Recently, the novel multifunctional S-adenosyl-1-methionine (SAM)-dependent enzyme LepI, located in the PKS-NRPS gene cluster for leporin biosynthesis, was characterized in Aspergillus flavus. LepI is considered as a SAM-dependent methyltransferase that can catalyze stereoselective dehydration via three pericyclic transformational processes: intramolecular Diels-Alder and hetero-Diels-Alder reactions and a retro-Claisen rearrangement. The overall structure was found to be largely similar to that of SAM-dependent enzymes,28–31 exhibiting a core α/β fold of alternating β strands (β1–β7) and α helices (α1–α19). This structure exhibiting α helices and β sheets comprises an all-helix amino-terminal domain (NTD), a carboxy-terminal domain including a substrate-binding site, and a SAM-binding site, which is formed by a seven-stranded β sheet rounded with five helices.

To better understand the mechanism underlying LepI inhibition by SAH, we determined the structure of SAH-bound LepI at a 2.7 Å resolution. The overall architectures of SAM/MTA-bound LepI and SAH-bound LepI seemed similar. SAM or SAH binding with the enzyme occurs at the inner surface of the pocket and is primarily mediated via ionic bonds, hydrogen bonds and π–π interactions. No hydrogen bonds form between Leu292 or Ile293 and SAH because of the absence of a methyl group, which decreases the binding affinity between the region (amino-acid residues 291–296) and SAH. However, based on structural observation, one additional salt bond appears to form between Arg291 and SAH. The close similarity between these two complexes revealed that the reactivity of LepI might result from the hydrogen bonding and positively charged nature of SAM vs SAH, but not related to structural reason. Although SAH-mediated LepI inhibition probably proceeds via the failure of a stable interaction between SAH and LepI. Overall, the present results suggest that SAM may stabilize one active state among many available LepI conformations through substrate mimicry, thereby activating the pericyclic reaction; however, SAH cannot completely activate the pericyclic reaction of LepI because it lacks of sulfonium moiety for catalysis, whereas MTA occupies the substrate site.

>METVAAIKTLIQQLAQSTDQFGRAEINDALRELQYSLETPFDTVMRMSLDTCQVAVARIGSDLGLFKHLSQCASPQSAEELADHLGCGRELMSRLLRYMASVRMVQQTDDIKYISSNITQTLAVPGLEAGMRHAFENLWPVLMALPDFLAERKYPDIVDAKDTAFQKAFNTDQDCFHWLATQPTRIANFKVLLTDERTPNFLSTFPLEKELGSWSAEPEKALFVDIGGGMGHACIRLREKYPNQPGRVILQDLPPVLQAAQATLPLSGIESMPHNFHTPQPVQGAKFYFLRLILRDFPDHQALEILQNIVPAMDAESRIVIDDGVPPEKGARWAETGTDICIMSALGSKERTQRQWEELAAKAGLQLQALYQYTWPVVNAAMVFSLQ[2x]>[2x]MESCYNPGLDGIIEYDDFKLNSSIVEPKEPAPETADGPYLVIVEQPKQRGFRFRYGCEGPSHGGLPGASSEKGRKTYPTVKICNYEGPAKIEVDLVTHSDPPRAHAHSLVGKQCSELGICAVSVGPKDMTAQFNNLGVLHVTKKNMMGTMIQKLQRQRLRSRPQGLTEAEQRELEQEAKELKKVMDLSIVRLRFSAFLRASDGSFSLPLKPVISQPIHDSKSPGASNLKISRMDKTAGSVRGGDEVYLLCDKVQKDDIEVRFYEDDENGWQAFGDFSPTDVHKQYAIVFRTPPYHKMKIERPVTVFLQLKRKRGGDVSDSKQFTYYPLVEDKEEVQRKRRKALPTFSQPFGGGSHMGGGSGGAAGGYGGAGGGGSLGFFPSSLAYSPYQSGAGPMGCY

Mammalian NF-κB is assembled combinatorially from five subunits, p50/NF-κB1, p52/NF-κB2, RelA/p65, c-Rel, and RelB, into homo- and heterodimers which bind to specific DNA sequences, known as κB site or κB DNA. The DD alone mediates protein homo- and heterodimerization; the NTD and DD together are responsible for DNA binding; and the NLS region is flexible in solution and together with the DD forms the binding sites for the inhibitor of NF-κB (IκB) proteins. The mammalian NF-κB p52:p52 homodimer together with its cofactor Bcl3 activates transcription of κB sites with a central G/C base pair (bp), while it is inactive toward κB sites with a central A/T bp. The p50 and p52 subunits bind to a 5 bp half-site (5′-GGGNN-3′), while the RelA and c-Rel subunits prefer a 4 bp half-site (5′-NNCC-3′).

We mutated the central and flanking bps to generate PSel (mutant A/T-centric) (5′-GGGGTAACCCC-3′) and (−1/+1 swap) (5′-GGGGAGTCCCC-3′) DNAs. PSel (mutant A/T-centric) showed twofold reduced reporter activity, while both PSel (−1/+1 swap) and MHC-κB showed drastically reduced transcriptional activity as compared to the natural PSel-κB. However, compared to previously known structures of NF-κB-DNA complexes, two striking differences are observed. One is that all three PSel-κB DNAs exhibited a distinct widening of the minor groove at the two base-steps around the central position 0 (−1 to 0 and 0 to +1), with width of ~7.5 Å (Figure 1E–G1). Throughout our simulations PSel (natural G/C-centric) largely maintained its widened minor groove at the central 0 position, while the minor groove in PSel (mutant A/T-centric) narrowed slightly; PSel (−1/+1 swap) displayed a significantly narrowed minor groove, which became similar to that of MHC-κB DNA recorded in the simulations. The swap of T and A at ±1 positions reverses the geometric conformation of bps at both positions. The thymines at both positions slide and tilt toward the minor groove simultaneously, narrowing the central minor grooves. Comparison of MD simulations and crystal structures suggests that upon binding to p52, the −1/+1 swap DNA experiences more disruptive conformational change than the natural G/C-centric PSel-κB. Unlike the natural G/C-centric DNA, the binding on both strands of −1/+1 swap DNA draws the bound thymine in the opposite directions of the minor groove, breaking the intra-bp H-bonds and severely distorting the central bps. Upon p52:p52 homodimer binding, the central minor grooves of all three DNAs narrowed, resulting in a consistent trend as seen in the free form. Adapting to the width of the DNA central minor groove, the p52:p52 subunits bound to −1/+1 swap DNA adopt a closed conformation where the two segments bound to the central minor groove appear to clamp the DNA, in contrast to their more open conformation when bound to the natural G/C-centric DNA; the p52 subunits bound to the mutant A/T-centric DNA fall in between the aforementioned two types of conformations.>[2x]ALTAKHRPSVVWLHNAECTGCTEAAIRTIKPYIDALILDTISLDYQETIMAAAGEAAEAALHQALEGKDGYYLVVEGGLPTIDGGQWGMVAGHPMIETTKKAAAKAKGIICIGTCSAYGGVQKAKPNPSQAKGVSEALGVKTINIPGCPPNPINFVGAVVHVLTKGIP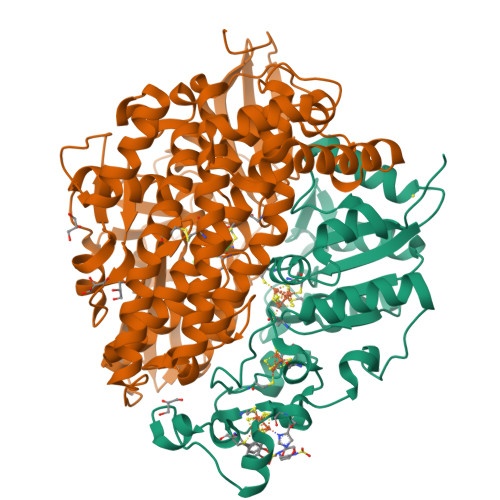DLDENGRPKLFYGELVHDNCPRLPHFEASEFAPSFDSEEAKKGFCLYELGCKGPVTYNNCPKVLFNQVNWPVQAGHPCLGCSEPDFWDTMTPFYEQG;>ASWSHPQFEKGASGAAESKPTPQSTFTGPIVVDPITRIEGHLRIMVEVENGKVKDAWSSSQLFRGLEIILKGRDPRDAQHFTQRACGVCTYVHALASSRCVDDAVKVSIPANARMMRNLVMASQYLHDHLVHFYHAHALDWVDVTAALKADPNKAAKLAASIAPARPGNSAKALKAVQDKLKAFVESGQLGIFTNAYFLGGHKAYYLPPEVDLIATAHYLEALHMQVKAASAMAILGGKNPHTQFTVVGGCSNYQGLTKDPLANYLALSKEVCQFVNECYIPDLLAVAGFYKDWGGIGGTSNYLAFGEFATDDSSPEKHLATSQFPSGVITGRDLGKVDNVDLGAIYEDVKYSWYAPGGDGKHPYDGVTDPKYTKLDDKDHYSWMKAPRYKGKAMEVGPLARTFIAYAKGQPDFKKVVDMVLGKLSVPATALHSTLGRTAARGIETAIVCANMEKWIKEMADSGAKDNTLCAKWEMPEESKGVGLADAPRGALSHWIRIKGKKIDNFQLVVPSTWNLGPRGAQGDKSPVEEALIGTPIADPKRPVEILRTVHAFDPCIACGVH[2x]>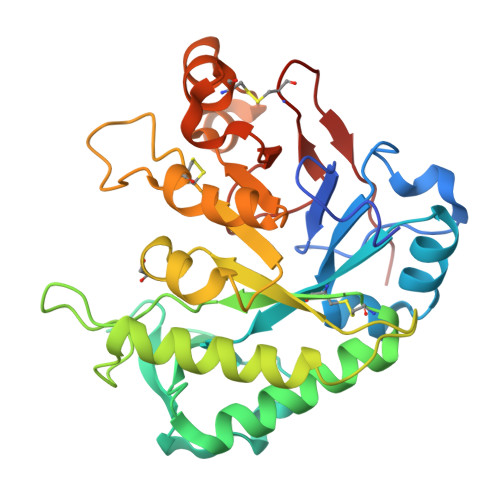[3x]KPATAARATGLADFKPGVQWEICIHHPIKHDSAADLIPTKAKVWDIDMGHAQEFPNMIPMLKSAGKFVICYFNAGALQDWDDDKSKFPKEVIGHSLSYPYDSEEWYLDIRDSRVLELQTARLDIAAKIGCDAVDPDNVDAWQQDDEDPTGFKLKSSDYTNYLKNLAKYAHSIKTKDGQPLLVGQKNAPEIAEDLVSTLDFAVLESCRGNSDPNEESWPFCEDFQTYIDAGKPVLQIEYPPSVEKTGKVSASDNKYYCTAEDEDKGFSKIIKWASAQLDGWGQYCGEEPFRTPAAKY> MGSSLRPLYMDVQATTPLDPRVLDAMLPYLINYYGNPHSRTHAYGWESEAAMERARQQVASLIGADPREIIFTSGATESNNIAIKGVARFYRSRKKHLITTQTEHKCVLDSCRSLEAEGFQVTYLPVQKSGIIDLKELEAAIQPDTSLVSVMTVNNEIGVKQPIAEIGRICSSRKVYFHTDAAQAVGKIPLDVNDMKIDLMSISGHKIYGPKGVGAIYIRRRPRVRVEALQSGGGQERGMRSGTVPTPLVVGLGAACEVAQQEMEYDHKRISKLSERLIQNIMKSLPDVVMNGDPKHHYPGCINLSFAYVEGESLLMALKDVALSSGSACTSASLEPSYVLRAIGTDEDLAHSSIRFGIGRFTTEEEVDYTVEKCIQHVKRLREMSPLWEMVQDGIDLKSIKWTQH;> MAASSRAQVLALYRAMLRESKRFSAYNYRTYAVRRIRDAFRENKNVKDPVEIQTLVNKAKRDLGVIRRQVHIGQLYSTDKLIIENRDMPRT;> STIEERVKKIIGEQLGVKQEEVTNNASFVEDLGADSLDTVELVMALEEEFDTEIPDEEAEKITTVQAAIDYINGHQA;> MAYHKKVVDHYENPRNVGSLDKTSKNVGTGLVGAPACGDVMKLQIQVDEKGKIVDARFKTFGCGSAIASSSLATEWVKGKTVEEALTIKNTDIAKELCLPPVKLHCS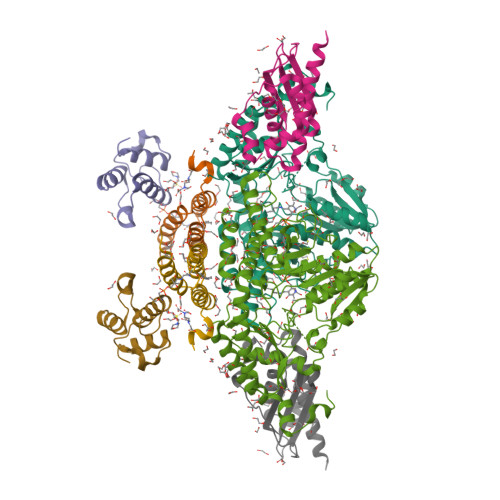ILAEDAIKAALADYKLKQEPKKGEAEKKLEHHHHHH> M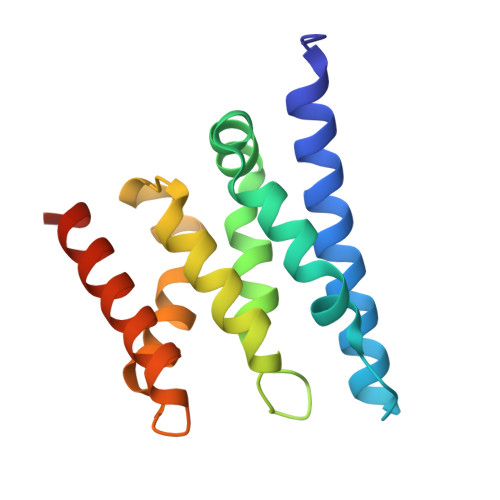DPGTVLEISRSLKKRMQDILKKDNANNLEGRPATGKIENVEEISDILMSKALQESLLDEGILDEIKGWLEPLPDKSMPNIKIRKRLLDVLKTMKIHKEHLVTSGVGKIVYFYSINPKESKEVRASAKALVQKWTNEVFKPEGGD> SNISRQAYADMFGPTVGDKVRLADTELWIEVEDDLTTYGEEVKFGGGKVIRDGMGQGQMLAADCVDLVLTNALIVDHWGIVKADIGVKDGRIFAIGKAGNPDIQPNVTIPIGAATEVIAAEGKIVTAGGIDTHI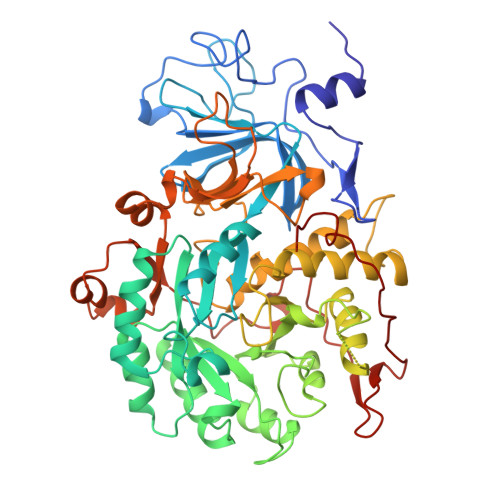HWICPQQAEEALVSGVTTMVGGGTGPAAGTHATTCTPGPWYISRMLQAADSLPVNIGLLGKGNVSQPDALREQVAAGVIGLCIHEDWGATPAAIDCALTVADEMDIQVALHSDTLNESGFVEDTLAAIGGRTIHTFHTEGAGGGHAPDIITACAHPNILPSSTNPTLPYTLNTIDEHLDMLMVCHHLDPDIAEDVAFAESRIRRETIAAEDVLHDLGAFSLTSSDSQAMGRVGEVILRTWQVAHRMKVQRGALAEETGDNDNFRVKRYIAKYTINPALTHGIAHEVGSIEVGKLADLVVWSPAFFGVKPATVIKGGMIAIAPMGDINASIPTPQPVHYRPMFGALGSARHHCRLTFLSQAAAANGVAERLNLRSAIAVVKGCRTVQKADMVHNSLQPNITVDAQTYEVRVDGELITSEPADVLPMAQRYFLF> MLKCSLCYLASKVTAGNAKNQAGHPRRKAKLFHVVPGTPVTPFEKLKEQRRRFGQDRHSRLPEYRPGNNVRMDPNTYTLYATKKGVMTIRESRINPKYKWLDVEPDIQKVYRSRELRRALQEREMASMAVGENSNYRVELDLLLEPDWRERVMHVPKATERFKDPNLFTRGVVNELSPLDRYSYT;> MLRNTDVRLFSTFALNPETSVAPHGPPRGLVNRYVSMGLPPWAAWCNKVNRYSLYRMSGVTQRSFLPKPPQEMDVIWLNERVRERVRTSRQVQNVYRQLKYPYVKTGIHYSDVLDHWVQVPMVEAAMFEVEKDGGFDNFILKRSGPELRSTYGERIRRHILVRQKEIQKNFVLQKQAQMLVESMEKEILPMEDGKKVEEVLEKYGIDKEQLLRDIARAAVAKKQQLASAVPQPSHVEVSTN;> MQRNLTKLSAAAFYEFVDNNFLNNKRPPVPGGSWTVEVLRNKSLADLQHIWFLLLKERNMLKSMKEHYLRHQEELGAMPAPSRLKMIDESMRNIKRVVKERDEEATARAVEIFKERLKRGIYRYPPGPPPPPGAHDKTSVVKVELSCYVEEERLRELFGRYDVFEPHKGIVRVELKLPDEVLKQKEEAEQLWTQYMAECSDVKAYHQWSTAAPSAYDYTEVELAPGIFANDAISDKGGKHSGDTETHEGVIVAARVPVPPPKEKQPPPKNPLERLKAERRSYLARTTIQLGYFPNVTLPPPRYETVEAVPRPVHPDEIEGPWEAYITYDREDGLSYAQSLGITTIGVATVLGLTEHVREPQPYAVVDPVYCEALRRERAREETLMKWPHVPEWKYEYSTYTRKHLADIVQYNYTNVVDYVDREVLLTGKSVWECPIHIDHTCGGSKTVPPHAKKPVRYMDAGIANVGVTDI;> MMRRMWVPTFSAQQQHLHHAMVLKMSTYASTPSGNGVTSAASNEEMNLHDAAAIAPGPYRRVGNIFIVHCDDHPFKHSWEVNRMLRELRLEFKGQTTIVPDIPQVRKRIWRVRHIVKVDVLDLDEAKALIGVPEHISFTDLASQLPPSFGRVKAVPSPVIRSKMNFMKLRRMRLRDVLHRDALELRLLELKRSAMKNAEQQKHAQKDERTDNKEGEKC;> MVLHKWAVVSRSAPPPRGLRPIARTIPTHPRLRPVDYKIPYVLRTFIKDRHTSEVQHLENRGMFAEELSIERSRFPRFHSTFTIQTDGSLNEREFEFAVPPIVTLFHDRLSAHRERQLELAKIGKLRKERNWETEQKGEESVSMACNALAFPYCIPKNMLKRSRVVDPLNSKSSTQGVTSGGG;> MFRRTFFTPMIAQPTLLMLGNKGGTPKRKKNPMQLRRKVYGLHFKEKYLKMEEWYYCPLCAEPKKPGEWCRREDCRQIKP;> MLSSTALLLRGQYKTRLKKRMVGFIPKVIPRKIKNNMVALRSEANTGHMEGYLKTETERLDATGRKVQKVLWDPVLQRHCLFKETKIKGPFMTKSAIAKKVDFPIGGAEKMLKK;> MGSEESNNICAYKRTISLAKIYIVLLVKTAMLRYSRLCFPKMGCEEITRKARRVQLQPTEYLAQHRMQVWQLRFKEMGPPFSRVWVALGGKMRRRRVGRQVDVKDMRYYWRPIEPQYQRLYMSRLRIRDHSNKLRQPMRLRATNADIGSGSSSIEWERASNRKYGAMLAPPKRQDFEFRVV;> MRGTTKPMLFLCSTAVRLNFFPLGLSAGPLNSHILLPRNNFDGRTTHGMKKIQGQSKDPQMVMSRDELKLRCEYCRFEWIHDTLCVRCPAQPSHDQREMWLHSTWMWGKQQPYKYYKYMPAVRNPRTGMPMAREDARSMNNERRGQGLTTRTLNLEKERRGISRDVSRIGQYNTRWKTRFPFPT;> AAAAAAAAAAAAAAAAAAAAAAAAAAAAAAAAAAAAAAAAAAAAAAAAAAAAAAAA;>AAAAAAAAAAAAAAAAAAAAAAAAAAAA[2x];> MRSLIAMRRRFVSGTWTIAVSTQQRHRSGSGPGDKRIRTDWYRCYPSLMREKDRDMYHCYYPYLFDHGDKMSLYPKIPENPREWQPEQLQTTYDAIREDKYDAFIRLREKFPELYQDTRAWDNPPPFGEFNMFYSVRFGMVGVKAFTCKDYDELGNQFDCTAFWFPDNQVVKHSTRNGEVGTDKVYVGAMNVPVEFHKPHVAAFYKAAGVPVKHVCAGFPITPDAYAPVGTKLDVRHFKPGQEVTITFQNTDYGFRGVMFRHGFDGGYVWLGDSRWQRRPGAMGTEGQKRIYPGHRMAGQTGAAAETYQGVPVWRIDYKNSLIYLPTLLDADVGTYVRFSDTINTKGLTLWNEHRGLPAFPTFIPPEDEDLSKLATDECQLKSPPLYMYFRDEFPATQLVSQADVEDAKSAKPATAPPKKKVYDMKKYYEARKKYRQSMQKARKYKLMGLRTKAHEKQEEARRAKILKYKRMK;> MRRVSFSVVLATFGKRHSSIFSPRYDWRTSGVHDIAPRDEGDFLYQGPQHVLPGAHPLPLHHPHNTITRPVISPYIPSPQRSHPYFTAPLPELPHFSTTKPIVYTYGTMKERIIAPVFNLKNEVIYTRELDPFIFGMYPEVEELSKNLTYWMVRCQNFASKWDYETREIWRKAKKNWPNTGMGMPRVGNRKNHLYTWGGRTKPSKPWNMLMPTMDVKTWSKSNRMMLTLKMLQGRLQVVDRLTLEEPTQECYLELCRNMSWDVRHTGGGVLFMDGGSRITPSSEFDRAFFFGSFFNGRNKIVRPTVLCDEQYDYNKTAAKQRMKGPKGAKNPIPINRFNAYDAMKHDRLVITEGALMQLEDELYEHKLQILPPHIRNQLPEYGYLDSEALGDCVPSLKTIQMEAAARTEEAESDMYKSFIDNPYNPWKDNMDASYAVDGADGTVQKFVDGKKVSWSMLS;> AAAAAAAAAAAAAAAAAAAAAAAAAAA;> MRRTVVQRVAPWVPPPRHDIKVTMPPPPGGEVGGRFGVSQGYSDRLARTPYWKRMALSTYKLRMMENATRYPMSEHRPGEYDIRYLPTPYPCTIRNRPLLEVGEPRQIPSIRIPVIFLVNLFDEAKGCWFGRRYETVYVERQFMREELMPQRYAIYATPEAYKLLGLPVVNHHTHEEIPKTPREYEKLLERQRYDEERWKYTIEYLFRKYEDGPPELLDRPEDGWDGSEEIALSSVAGAGRDGVVSQRKGPVKQRKARKIKLF;> MSPASPLPVAALSRLRITHRSFLTRSRGRHVCRSAVGVEYRPEQQKKVLDHSYARVINAEVVHGDEQKFWGERRTFYTQRNIFFPMWDRCAQALILITREVPRVPQEMAFRLMAVFLKLMLLPRLMMNTELMLPMWIASNAEGAMAAAKDGSKGKEQSSKQQGESKDDAKKEGDNTK;> MLRACGVLQLRARPKTVCVEPGSNRLPEALVVEKARDIFGRPEFPGKRVLHNWRFFIKAGKAATGPPVGQEFSKLGLKAMDFAKVFNDRTKPHFKEDVELIVRIQVYFDKSYLFTIEPPPTAWFILRALRKKRRETGPVPLRGHYCALMTLEMAYEIAKMKPLCWGRPEYPLLETRVRRVVGQARRMGVCFIGVDTPYSSPVKDMTEQQYTEECERYRRIHMEQYTTLRQRELEEAPLIERLHRPNMSPLTDEQIEEGLRDPCLLDTLWRASHPLSPYHRDLRERELARRYLNARGWVKDMTPEEMRIVFMNYRLPEGEKRKQMDEAAMSGEVYWTRDGAQL;> MQRSTRIVMAPFKSVLRRHKHHPEGLPLYNDMSKQWLCREGERWWLLDARGEQLPRVAAVAAQYITGQHRPDFTPGMITGDHVVIVNIKDVVMVGDQWIRVPITWQTAYPGGKYRIRLTDMYERDPCMLMWWFLKDEVNRHFVRKLKTRIAPLEKAWLYEDSIHPHADKNPRPLCWTDPEVKGWKYRDPQFIRRWKPNEFMH;> MLSVSPPLRRYRLFHPRREAIPMHMCPAKTIFPLINSNNLLVKTRNSWEDFTGRKEFDEDHPLPVVGSRLNGRTTQHKWNHWDQYLNPQITQSIKDLTPTPEYVGMRCGHNMIKMGWMKIGGSWKYSRGYNDRRRVFARGQWQERKMTPRFMLAPRVSAGGPRNRYEGKLVFSPLRLSKLLWAIDTGRINPNEVITLYHLRQANVVGEREIVWPGFVLISNGVRRVPYPIHIELQNASAESIRLIEEAGGSFTCVYMTHEGLYQELHPEEYPIFMDQELPERRGLESLATNPSKRGWLTRWYEDSSKYAHPAAGRRYSHYLKPPTERDFPATVEEYEMVKHHQKWHLNQPGTGTLLPWHSYNTADLVKRAAGRL;> MPSPFQQTLLARAYHYVHPKTGRPIRQFRRYGDPRYINNEAALIRGQWGLITADFGMVTQSQMENARLAILRRLPRGSFTLTMHTDYEEFPVVKKSPESRMGAGKANIHHFAFKFTTGVPLFEIMPISARRLNQAEAEGIFLAGRPFIPLQTVVVPQGRVDEYHVFK;> MLRITLLVVGRAPPVIGCTRKARYAGIDDNPTITYKPWDTTEPLMADYGWTRGKLPKFRARSPFHRQQIARRMVTEMIRKDYCIVGGARAPALRILADHVVELAKAGDTDSRQQLAYFLHDPLMVDKAFDEYPRRFKDMNAKYAMMTRLKSRRRTDAVAMYFVEYKNRDMSDNHKGEDYSAGPERFFLPPRIVETEKGIQRPPHMQMAFDRWASKFKTEEFHHWWRLRHAKLRYWGVRNVPHPSDVDPLWTEKEEEEWHNEMLANTGEYEDLDLDDESYTAAGEGGEPSPAGDGPQPQRVG;> MGYTRERTNRHFFVARANAFFSRLPIARVQRSLAMEAVREGRMRPWKYTKEQILGAPVTCNFEYNPRPVRLIGTVMDAHTEETSIKGGLKVYARNEETNMMLWIPPGNPKLRHEVTSTKGSFQHYLDERDKWDEAWITGRARMK;> MLRRTVCVQHYRAKLELDRIRSMLRGRARLERKVGLKRLFFLMRTQTRYRVEQQAHWERAIVRKNVDSAAREHGTGWQHLRNELGRQNVMLLPRSQQLLAQYEPLAFRAVVELCASRIPPPPPPVVASVPEESYTLWPPASHDNSECASTDGSDAPHGQQQSLSHPAARVELRCGVERVLRRGPSGLGNNVNELIDAWKEFDVSPLRKGEVNK;> MPSLANGLRCPDALITRTLNPLLNGPKFAVIYCGNHQYKVAVGDVIAVQRLRVEIGSHIALKKVLMVGGPRFTAIGRPLLEGVRVTAQVEEQKRMRNVVSLFATPGRRHVRWVDAPHAATIIRICEIFYSPNVVGELDKYKGELLETFTPGQHTNPVYPVDDGYDVFRKKDKEAMENATTFLDLLGGV;> MPRPAPRFAMGHMLPHRSNVGSQFLHTQRHGSRSTWYKKHYFSLRPFAIQRHHGTTPRILLDRSLWKSLWITKLQLPDINRWERVVNSRRVTEDRYAFVEEEGVMHKVNWGLYCERLETELTVTQERLPQHTLLMKAVPSSWKKLDIDISVIRGLSLREAMAQCKLSLRKGHQIVFRALEMAQQGAEAKGLDKEHLRVAHISCYPGPTDKQIDIRSKGYYAWKTKKSSHLVLTLAEDPEMVLPDRTCLPYSSLMSMKRAGLSAQPTVIDVPAITADGI;> MVVSLRRFHSYANSSRGGATTCLITGGGKGHFALTVSTRGRFYRPLVDDGINLWRRRMGRIHKGWRTWEYQHTRPDPRPFPDPPVNDYFGRSRIWNPIACKLGYVRKKADEWGWPNKPPPPTGLRHSQEFFPFFFERYFPDAEVRLLLDSVLNNETKRPVFQIPCSMSKVELVNYLKNIYGIDNVVRVEVRNRRGRRYKNEVGEIKMMDDYKVAVVELDTPVSVELKQIKGTEDTSDNRPQERITQ;> MYARFRTRSKFYFRPARPALAYNVDPNVMRRPKVKRGLLKGTYSDETVDLRDRERLELLESMRHPRERDFYQDHTYHNQWLRRDLEKHQKQQLAARYKYFAPDFEISPWIWYPGDIVEVVSGEGIGQRGTIIAVIKYKNEIVVQNINVQDVVIPASESRPEQIVQREHPISVTRVRHVDPSTNEICNIEMVKVRNKETGEMEEKRMSLESGILMSIPPVNDELEVGDPLKDTPIQDADEATYDREAEQAVLVDKRLEAMEEHFVQSLKQSYEFHEPLRRKNAEDMRQFQTDVIDMACAMLGERLLDTVNASDTSSFPAEWQEAIAMHVEEIEAEMEEVAAKEMAEAKEGGAAENEQHDDDLDDDEDELDTSEESVKHV;> MVMRRCSYNVHPTWYMMPLRAYHMPGWKTKVSTKDVRTREQREADRKVRQIEKLPRPQALHDFQYPYEKTVLSDTMFQYPVYENELDTPHLFNITEPPDFFVYWNVSDFERTSYPPLPEEDHRLLLPLSGSAPWKQHRKRSLKYLRKHEILPNYLPHVRQDVNLSVVFPGVYATRARLCEETGEPLPPPPPVSRMTHRNFWMTAHCGNYIELADLQHPPSIFFLDTVSATGQGKAVEKDATEEGSDEVWYTLIIASPDYPFRVPASVDASTQRGFFLNYMMSNLKGGGNSTVLEEYESEQRQNNQKRQHLEELVRNPAPIAKEGDVIVSYTPPLPTEDAGTTRHICMLFKQRSYVSGASCALDDSKASFAARANFRLHAQHRDGIPSSSVEMLSRIEQVLPPDPSAVTFFQTKWDIQVQEFYESRGMLEPAAPLDEEIEAILAYHARKPSELRVRARHRPDGSTNVGDDPNFWAQAEPTRMMDGSMLSLWSRRTTLGANGVPITYRR;> MVLPRKLVGQCCLLLQKKQTAASYMANAGKVGNEEKWAQAAMEYLHEKRHCNDSRKRQHDVDNERRMAFAFDRYCSVNEKIFTERLSRLSDRMTEALETIKQLGMDHALEEALMLSSEQPPLNFRRPTLTPPVAGYEPGFGLDVPQLRSRQAEYPPVGRPTDAMEFGEEKDPSFPLVESFRVEDLTTQCLNELEERHGEIREAAPTTGVEGEAWEAYVALQKKALARQQLIFELCNNGELRERYDSDVAFRQRVWEERGMLPLEIERERLHEEPRHYAQEPAYHPFRKM;> MLRCSCACRRGVYHNAPSVYPFVKPFHDTPYDQDRGRHDSVGQRYRKNSWPEWMDNGADGTGYGIGLHRTHPLSRLRGNLKRSPSHVPRVLGMMIQGVWHKSGVKLYFRGGKPPNPSVHPYLTGEPCPLYGWKVTDESVIRQFNMPSIDGTNFRYKPYVALQERKIMGVQVPSDSVSLASGRTTESKPLAKRLFFWR;> MLRLCRVSLRVQSHQKKRAQHPNAGTRFGRVYNRGFIRYGFGGFGMSVYTPKKDRRFRVQPLPSLHANSLADDTPLVTTTRTLSPNFRAFALQDGGVFFTHPSHEQVMRVGQNILAEETKATGMTSMDTYVNSRIQSIIAENTVENVALSHWRRRHMWNLVRTHGKLQRHWGVSDATKGARSNIYGRPS;> MSRNGELCLKKVIISYCPSNGAPNTRQFLATHLPHFHAKYPSVSIDLRPRLWPEMAITGVYRDGSERSYNTKNLSPMGIFLRLNNLVSTANDYDQPFCASHLHFQRRSVQGTWNPWLWNYETERRRTEAPQWRRKLSEKEWDYYVGQYSAQMKQEEDEIQRRVADRTCVQEQSTREVQERWKRHVVPRMQTDLEFNLSHFKRQHARGQLQQRPVTMGEYRLFSVPDPRELGQDAVDTMRRRESHNMEVWWRKRKEQLKPP;> MRPVARLPLSRVLSGCRGFHSQHRTPVLPQVPAAEVQQAASESKVRVAYLLHRQPVVKPTPHPLEMEMAFLLQREHQRYSRHESSESATHFMAQRGQSIDALNRTDPRQIQSNFFGLELYQDAMRVVLQRYKPERRVTPRDLWDPATYGSSNANSNASSPPTRHSLHRKLDDYLHLIVRDEASGKWTVPQTELRGRETLRMAAERAIATDNGEGLDCYVWSNAPQATVPNANDGSWLFIYVATYLSGRPKFSEFRPKTIDHAWVTRHEMMQYEENFQSPELVRVLLDISADSTFES;> MLNRSRLRRVWLGGTAANTSLGRDVMPSTGKYINIVSPTDVAANISAGAMPPEANVAAALPVPRIQYSKWNRALRSDVYDELLKLPLRYKLHDFAKLCPPQRCQEEPEAVGVVGRDSAVGYLPPLGPADPLDTIPFFVHRSSNGVLPGKVFSMHPRNLMPAFYLRIQQVEGDMFRFEEELLKIFPTKKIFVRSHSIYVYNVALDGRMVLHHWLLGLGF;> MRLHTVRAPIITRAAMRGYSEARSNYDGTSLPAWPAPGKKPTYPAALSELRLPQPRMRKTRTEWMYYHGHGGCPGKYGPSREIADFEYADGTPASISGRRFAFKHHQDHLLVQLIRAAATVERYDASGLLPRIPGTAEQRNWDPAIPLFLDDVDEQGRPAPLRTAGDAPGTMVSHVCSRVVDERMGTPTHTPNELANRHEGETLEANTMFATNDPSAFVSDTVKLRDDKRPYWSRRRWALTDKFLVPKSPKPKNTIKDE;> MLNPPKHYSVESLRTVGLLPAQLALSRKPRLRPHVGNLKGLVYPLPYYAMWRGNHNKYTYNKSTVCLWGEGDTRSMYHQHYAHAKCPTDYGRGGREFEYLTVKRGKMLQKPLPRVQYVAEGSKPVWLFKSWHTPLSSPSMWEREVQYAEHTPEHIGAKRPLAVVAPRTMHRYLFLMHMEKVTITVSPLLFGYGHTIQKAVLDFYRRAISARSPFPKDKVFLFYAIDHITPRIEVTWLDGTSYVPPVLEGASSQDLIQMVMEEAWLAADRMAAEGRVLNPLAIDDYKWDQLVVFKKVRDKEASKGGGRKK;> MLRHCTAHRRYRTAWRELLHPLPVRARKMEWLKRDAVEENEEILRRPYYTIKSYALPPAVGRQESIHNSNNIRGGMHSSHSLDLIMRQPRRVKTPEQLRALRDRLRFIGVTGPMPQATSVSTKSYTDTYGSRLRPRYPESWDTVPPHQPSRELL;> MLRGTRGFLAVSPGVGIAPETTPVKYTPMMLNIQNMMWWNGKRNLYRATYREKTWYEISRTGAFTKGRRPVMRQKYSREALQAALAMVPPGFEVADVPRPPQRILAQSEGIVGRWYSNYWTLHSMRYQCLLAGVEWPLGERQRPRTNYDEPFFFADFEESKAIRDYRSRWINVNRSLVGMTKRMKEAEEEARYMQFRKLQDTFWSNRKVLVNRVKSMYNQGARTSAKDMPIKTINIKAFLSE;> MLRRFALTSSVALRLRFERDSGHNTVRYRPIPESMQPKHLEDNFTPFPLPKFDESLEYGPVRLRNIPDIEAAKERRRGSRLAATEVLLQETLQEENQFATSGKGDGNMAIAITERHTEDVTTPAADSRFPSQTMSPCSHEEEMRGYVVSRDYPLIDRLHCTRSIEELVAQFEDRPQIESRVAALADMASTVSFRSDEELLRMFTAISAPFSVDGRGLNFLTVKVSKFGRPYYVPNSLLPAYVNLVDATTIALVREQPWRLSASPALFIQVLQFMALIKVFEPNKWFTFSDHAPSNRADYRHAIGVNHSTAFWGTGEELYDFMVELLRVEDDGRIPTMLDLCTREQMVDLLSGFCGVMPCGKAVGDVFKTITDAFLRRVRNDISGPWSAHDWAIVERMYLVTVLCDAGNNEILQLLLSDTASPRGPDFFAAVSRTKDTPTKKRALCLLQEAIDNASAKADKVTLLGLLESGSEFLLSLVDKGVAHTFATQNLFDYRILNSFLHCSLVADRLRVEQSVITSLIPSSLRDVQVQMLMSNERNALNPLTSSLPGNSGAIATAPKLKRPLMTMLSQLEYLNSIDSVFILHSSLMATSTDQLVSAVRRLPSGKDSLIVTMSCLRALSVKSLTSPSMKERIACARALEIVSYELEKGRAVLLPFSEEILLHDAGAYCDEDLMLWTVAAFLARELPLVKVHTLMHSNCTARTPYRFLKGGHNLLVSSRSLYDKGAPLLSSLHSKELRLVTHNVRLRTPVRDRKCTLQYYNPIRARFVYRRDKPLFDKYHVTARNLAPGFSRGALKHDWRALGVYTPDHPQVPYHPLQTWMLGETTVEAE;> MLYTRRLMTTGGSATADGAVSYSKGSYHIVPKKYTVGKRIAVRSYLDRNRTELSDRTYMPQKAWFEPYTPKKFDMEHQRISHNFYNLETKLIWTAFDTPELIGILLHDETIKGAPHLYDAEFLESAVHWTRESRYWRCIGITKPFYNKTTLRAQCWHDRGLQVGTLVFSQAMRDALMDLERAVRRKELGLEPNYVWDRWGPVGFIDGARTDHLPRFAHNPYVDPDGVEVTEVDIAPFNTHEQIKERYGAFIDPDLRPFEGVFRSSSSSSSSSSSSSSSSSSSSSSSSSSSSSSSSSSSSSSSSSSSSSSSSSSSSSSSSSSSSSSSSSSSSSSSSSSSSSSSSCDEKVEALRLMENTRHDAARVRTFYEEKCGFSDFMRTPDKVITAAVLCYLQELQRICTETDWGKPLARCLTDLERVNVMGKDAFLVYRHIEDAILDKKRRVWATRFAGEANEESTLDYLLENFGRRTEQTRNVGTTGTEFDREQEPIGRQVQRRVLDSDKASKLAEVRQKRGKMWSNKKSVFDSLHQKQLQNVTYGVH;> MLRRLAGCVAFRKNVVRPFMNSTALLSSPPAAVSAPVIPKSGNEGKDYSVASGSVDTPVLDQLVGYYVNIQSRKMYYKDFLRIEHQAVRWAFADIRKNSEALAHGLLQTGLRPGQRVLAIQPCNCETFVLQLACAKIGALLAVVPHHNISADKLRFYLNEFQPHHLIAREWIVVPEVKQGVLVERNMHFWDMIYNVIPELGLSYPGQRFQWVHSQEFFFLKKVVITDHNMNLLGVTPMRKMLVWGPFSYYEQRLRRLSALLHPDDPILALEDPHPALEDKLHITYSHRNCINAGFLFGNLMGLKAESRFGVMPNHHVDPVGAIVAPYAALTTGAVLVHIHSDMFTDDHAINGIEKLCVEEVVGMLGKKSDFDLLLRHAGNFDADQYEHLKWVVLFEDASEPTVGDEYLQKLAKELGLEDVFVFRGPLESAYMVMWRSLKRARWEMVPHVEAKVVGDRGTADARILAANTRGNLKLKGPHISAGYYNNAGLLTELVDERGFCSTSREAVMDERGQLTLHGTQLY;> MCLKRKAPHLFCFCLWSIFLSFRCFCFRSYAIMLPLLSFPTIQISIFLSFKLPITTFLLSPCFVFVFVFAIRYCGELTLNAQLVLFLLYHCAQTQRGPLKEGEMPICPGLCGELAAVPFRVFLGTLPTLAVEERFLRQLQPVFAWYSSRKRVKEQANEFIEIDLASCDAELLLRYSHIYYVRRQLFDELIERQMTLLDSGKAPKMAEPSLLQCLAGCNMTIADRLQLEIRQLGAAKRAASVPGRRELDPVARLEVYDYACMMRLVEEDAGAVGDAEMKARAYLPREVIESKLGHLTQLLLGSDARAALDKKDVKLLNRMIPPDYTRVGCVEKLRPFDVTAYFRFYGERINNVKVENYFKRALWGHVYRRFATTPSFLSGVSTYWARHSGLDASFTTTTMPQEVAVAVCDQQIQFPAIKFRAQYVYTSPETARQLWRTDAAVPLMRLFPLMGSRTAEDLAAGVLTDAFWMHLGLSEEENLLQDSLLLKVRRFVDEVGDMYETNIDSVLKRVDDNFKQVVPQLKAEDLQVDAPLQDGEGEDTVRETVAA;> MLFRSVSCKNYQRGGWSPGSKHQKHMTLNPTLYLYRFPGPHGPGPYTMKYWWTLGCFPTGMEVPFRLHEFLSTYQQEHVPVEVEEWLRCYIKDPLSELVNASNDFFKAVEVYPEVESARGYKTLQPSIAPLLVPMKKFEEQLGVKISPVGLRSVLSNPVLKDRFLDDLFDYKSYVEKGGSTPHRRLARSRFEGSLSVLGECEKCLPEQHQVEISESLGTFIGATVSPAETTADDERSLILLLTTISEGCINAGNYSDAASVLADALMFCHDPDSQATTHANISFASLLNADFKGAEYNGREAALLQPQVKPTSTACARGYVGWAAAAAYQDDFEKAEAIVKDGLTLYVGNEHLEKLANKLQALREEQPSVYKQVPRSLRESRSHLPSQQSRGLLSGSGKGFSNEFDWVEFKNKLYPSKMDPRNNEMGSVFRRVGDLGSFISTSRSMERL;> MSRSAFSSRGALLFSSAPLQCQRRWVTRLYTSYYTGVLYPNQLVQPKQRLPADVSVSAILQKRSEPEAAAERGSNKGDKVDVSKGEKTPRVSWDDADSTDVMRVDNTQQLKEAPQVERPYVPLGEVAKLELQGDYYMEGGMFQEALEHYGVVAKAYNYAYPENHAQRIGIRIKLSAAFRQTGRLESSLANIEEVLRMLDASTRPSLELICEALLELGITREALGMKREATEAYEEALEVVNSFHNWGESHRMLRLLPRLGRRFNYNFEEKFVYFSPFDYDRTFALVDQCLERAETIFNEIGDVEGAIRVLQQRKEMIDKKFFNMRDFAGRIHTMRGHWKRRAQHLTNAPTPDELLRYSPTIHQVHRDFKYELTAPIGREKEVMPGVNRLVLDMGNPYRRRGRLSNKMLKDADHKFANYVRQKEYNE;> MRLARTLHHVASATTGGGQMLEGLVNDGPEVAHKQHASFTPFSIQPWQARCVGASRRKLLPQMLMYHGARLGPRPLIILDHSTKGEAGVAEAARKYESILSQLSWDYGAVYIPLHAQCTDSSKDLLEQSCQRICAVMDALDVRWTHFLTYSYGALVAVRMASSQEFPHRVGTLMSLDTPLVTREFLRNMEQREDIAKAERDINVPEDGLAFAKQALLSSLEGPLPCPAAEDESLYRDYLFDPNRIFGAGGLVRDESRYVPLKSLLGVRHPVQLIVPSANPLSDAAAHSEVFGHRRPAVVKCCQRHEDLFKESAAKEVAGVLGAWMRRFEPDCFISKRYEQAANEMGQLMLSTAQVSSESAGKGGGEPRKKKEKKKSKA;> MLVPGLSLTRRAVTSSCCRPLHVVRGFSTTCTLFGLEQLQDVPTSTSRRPTGLHRGPGKRQTSEREAAQYKFIRRWELQMRDEWDQLEPFKGLPKPKRQFGNEAAEVIWPYALLLERVVKVHPFTKSIYVYYAQRQSTARGKLAAEIARSFAREFLIPITFHNSQVYTEAEMLLEYSETPWVVLHSLDNGQKPRILPVAPVEGTPAHTAVEQLLAEVVQGCEALGASVADPVTATRVLNERPLQNQYVRVDYQWFGDTPDERASHLVRWEFEPEQIEPKIRHRTRHVLDWLNYDGNLPTHRAVHVNAMREKARQKAPRTVAGPRTFYNSAGSRANARSSRFGGQAAVGK;> MLRRSDLLLKKGWTHNPGRTRRGGKNLAWRPKMSERTLEQFVPLHLAFPRRHPNSWQERQFHLLGYVKWPKEIGFYNAGDNFELTPQAAYRIYKQNCDETFWTRLHNEKTIIHLLPLVEQDPGTNMVLVDDIFRHHLKRFGADHYIYNAVMQAAAFAKDFPRCEQLLAEMRGLGLEPNAQSYVNMMLGARLTGKPRDQAEAFFREGIKTGAISAVMRLDTEFQMWMNQLERLGSFKAKVGYLSVNEEGASPMPRDMWALWGWHRTEAKFISRKQMISEQVQNRVRSGKELVGTVYQKARRQPWAKYNGMFPYDYNGPARRPAASFVDAPTPTHNAEVCGTAYA;> MLRLSSWNLKSQHHNVLRRSRPHIHKYRELNRWQRQAQGISKWDQSHSHRPLPYVERFNPESVGLTRGTSAFAWKWWHTQYPWLPNVPPEAAQIDEAQKQERRSHRPPAWDDEFAKVVLNMNDAEIREYLMSKLTDVIFLETQRDGYELRRLDFEGKPLTSLPEPRIIENFVLEEETIRERVIYQVVEGVFRLSPTSADRRELRSVANIIDYVLTHVRAARPTDRERRQERPITSAALAVMQKCPIQPQLGFVHALPHDTRDALLQEWERMHHLDWQFGKAVYTPRSKENVRGNLTWLREDRHYDQRMKFMQEVESGEARAKHMKLIAEAAGN;> MYVFRFHISSFHSFLVNFLQPSRGVGEPSRLLHHLETHPSYMRRVTSTAVHRTVSSVLSPALLPSFNGTLLLSVCFASCSAAPVRNLYKRLGLDHKATSEEVKAAYRQRALECHPDVVDDNQKAQAEVDFRAVSEAYDVLIDPQKRKEHDKALGLERTVPPAKKQQEGEGVGCDSKGSFNRGVTRPRNRKPFVRGDADRNFREAFHGMSLDQVLFRERLRQRRMQKQMEEKAKSSSSSSSSSSSSSSSSSSSSSSSSSSSSSSSSSSSSSSSSSSSSSSSSRDPQPPPSDYMPFRPFHGWTVPNGVRTPPEPTLGPTAKVEDVKDVQLAEPAVGDASHQRKLPKHFPVVQASDGSSLLREETIACMERERRLPHNMGKLYSYHRPY;> MGASAGLIRRGGGVFPDAVSLTLTPSRRVYGGSGRGDLLYENPDARRHSGRALGVLNGVRHSSQATMPESGQLYYRKLILHSRPPNGSCAGLQRHCHDTCNWSYLIPSLHRCAESAISAKLWEKMCQLGLEDRSKAWVNLTQYERQRVRDGQNLYRYEVHQRLPLLEESIGWAQLDDLLGWFR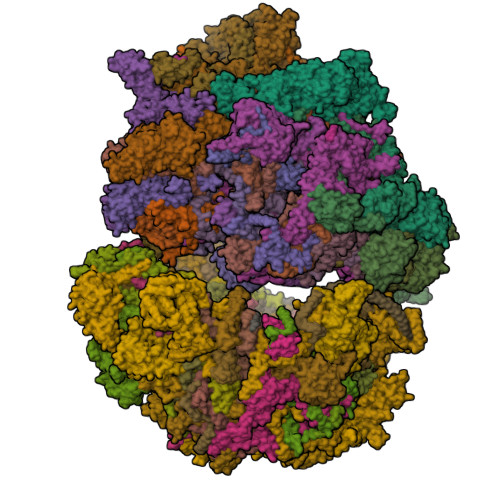SARRAWVRLPTSVTLSRESSEAGVASVVSPSSAMSCRLEGHADSRDTTPGRNQVFDTPERVEQLTEATVHRIREELQRLNRSERSDCEGSAAMRASARRLARDEELSRCVEEELGWHGVALQHRIPVPK;> MRPTFPALGSRAKGYENRVMVYAHRRHRAWYLPPKLAHARSPLANKSPDEYGNTWDPRTGVEWYHRLRRRGAYRHWPWARWNDDPVRQHQELSCRRTFSAAVTGANEGVPLWNYYAEVGQEYGLPSHFPLSFMAPFIHQYTSRAWSRKEIERHLKVVEERTGLRTIQQACDATSELLEWGEEEMGVVPHGLLQHVVMLAEDIVLQNKKKAYRKAAHERGILRTTTMERYYALPHLRTGPPMPTTLEQPSGEFPWGKFSTMVGGTRIHPLYRPDGFFKDNMYPA;> MCCLYTSDVFFWSSLVVSPLPRIVRCVSAPQIRSIPCGSGDFSVMKRSLIARWQSGVHTPHGVVYRGAKMKNWPEQRIPENFKFTEEQRFRTKAIPRDVGTIPRNFVLGVLYRHQPCEVGGLWEHCTNDPEIVLDSKRHLREVLKQAREEGFVTFERDAISNEWLCFLTRERYEEVQRIVTAKSEAVDSSSSSSSSSSSSSSSSSSSSSSSSSSSSSSHARRLEEEVANTTRYLRRFQQREIDYLPYTDLNGKVNFMWWYETRDVQQRADEVLTDSSSSKALAGEEEHKAGSQLEATTASTS;> MKRLFPSAGVSVVLTSSSIVMSCPCNHIFTSRRAYYWPYNEDFVPEGAETSRFQSSGSPGTRRRVLQEYALSPLFGARVPCCVVGTLRTAKEIIVLKRDIQSLLCELMELPQGSVTLGPLQQLREMMLYRHGTPLSPRLGDERQLNMDAYARRPIAARTMMDVFLAEDMSLDEIVNFGRLSLGKLQIALNNLRKENAEKSSADCEDGSAVEPAQLLVDRMGISYCEIPSLDESDYVFAEVGGVAVTDEEAERVAQRWAERCE;> MRRCAACLTSLPVSSPTGAAVGAPAAPLKTQAPSNRSLLGYPLRRAAAMEMLYGGICIQHLAQPPFPLRKIQSESLPPPSLQGERDDLELEVKDSTGNVMGYRLFPVNIGIRARTESVRVRSEDCYKRFLAQKHCAAAGVPLQFPAPSSITNSNCLATPRAASHFHPPSSSLSLFTRPADSQGGDVGRTTPADVAAYHPRAWRPYQMLKPMPHNWGPAVRSSGVRGPHMQLLQERIDKKGFGWKRKSRSLWQQDISTAGFRPKRYF;> MLHRTRLAQLINGRILQYFVPYERDEVNPVVFMDVTVEGDALGRVSVELFHDIVPKTTENFRSLCTGERGYSQCPLFYKGIPFHRVIPGFIVQGGDILLKDGRGNVSVFGFPFPDESFEGKAGKHLRGTVAMAHSAPNQNGSQFFFNLARNDHLDGKFVVCGQVIDGWEVVDRVAVLSGSSCGTPVSRAWITECGQSSGDKLEDTERALSGERALHTMPGKEVLDILSPRY;> MLRFTRLFREMAPELQLEYMPVLFTRTILGPQGGFAGEERLVKLEVARKYMEAGHAVTPTEELRRGLWCYNPDTDKYDCFIERNEEFLDFAARKRQWLDVYWRVNTGYLLFGRQSWGQGFLINCPLRKRDVAQKLWEQYKVRIDPRLIEFREKDRRTGIQELGHNWCWLYLPGAEELGINREVYDNKRVKVRIHVRKMNSMFALY;> MRRLGVFCRGQRNSPLLTRGIATGGRVTNEDRRWWLVHLECAPDITPGTFIAWLDCCGTHTCKKLIERNIWTIEQVAALDSDQVDELKYREGCLKMDVVWEHARTIITPLRQREVTGGVESELQGRIMELRKKRELERRREEILKERANVSEQREETLRK;> MRRCIPARGGFTMKYKKGTGLWDEDHVNDYKTNRYLSARATMRWYQEMERHQTRNSLNARRATQSHNNNRGLHHTGRGAFERELERRGVQVEKYPLTTTTGTMRVAELVILRRMELEKRAEEALAEQRGELQKKNPTPSEWYDESKGPLNPNFLRSMRSHYEVDIANLPDTPLIRGQREFFIGEERGNGAA;> MLNPTFSLYRKTLQSYPVPPKIRHYDRRWSGSRTNPYNRQYWRVIMNENYSRPSFWVSDFRHRYLMRTGTDYQGQVPSSPQPGLYQGFSDVHKLLANHPKPQRESRHLPVLPMTPRIVFEHANEKRIDTAKRMRRDRRRIEELKTLEFWGWYMKLQRVRGRWCREQGVSSRGVYGPAVDAAELWG;> MLQINAFKLVRATPFLLKRTGKPADTPDYKQVYLPYDAAPTERELERERRRFKQAYHGRMEHRKLVEVKEVPLNVYTYGKEGMSLPIAIFKDQKDPVIGPEWTYPGIYENKIAAQHWYTEELFDKESKEAFESPWQQQILDNQVKRRMAKVMFRMRQVNMKAVDLFQKERGSSRRSGGAGEKGKDGGGKK;> MSGAFGCGSYRSVVAGTQNVPRRMTFYPSAYELIQLHKAHREVIRHFYVRDKIFDNKFPGNALANGLFKFVPNRRENYHMRELMESIRRRSIWMHRIKQQREINAKVVENMEVKYGKKAAASMLCFTTPDSNAYFAPHRYQDVANSWPNYWQHPSVNHVVPKPRWRRHRELGGITRVEDPFAVQASDY;> MLRSRIPCVVVTLVQCRAMHGKPTQSHKVRTQHSRRWWTQSKARHLTAMPHDECKSRPHFPAYNEDVDRPMVVPPDAICFNCDKPIDAGDVNSYVWIPAGNATVPTPQGYFFHFGCFKCNRCKYRLGHNKFYSKDGKAWCIPCALGRDVRVPTRRWHTSYVNTHRTGSRLTGHFFPRHSHQMEFLFDPNS;> MLFTRCLLAVTTINSSTASAAGRLIRIRKKSKWIDRRSKRIPHNGKDVWQFGEQPSCALCHVRFRFKQDYEAHKESELHQNRLRWVETMKWWEEIGEPHHQQHAASEWEWFRQRVLPAKAAAMGLSEEDAARELRRAVMHETPRWYSRIQPPNARSEIKEPRDQRWPSSPKW;> MRISERAFMDIAIGTKAPRRIVFKLFPRKCPSAVKNFIELCSGNVSTDTYESGNRDKLISESALPQLTYKNSTFHRVEKGYLIQGGDIVTGRGTEQLSIYGGTFSAPEEVRASVFDKPGLVGTASSSPNAHGSQFFILTAKEANHLNGTCICFGQVADGLDVVQEIEQVPIDPSGFPSLKVSIVDCGVLE;> FKQGQGMFSHQLKRLLQKKSIHRYNWDPLPMYDPRKLVHASRHMDVETWREVPDPHWDERSYLVPDQMFYNIPVPPEYKDAYWWRELQARRVQCPVEWVSHRMYNKGDRQRYDFQDLAFRKKFEFSYEEVVKNAKDMRS;> MAQWVPKTAWKVSNLNKRYGPGYITSGFSSENTLGYTHMVHDSHKLREKLSSRKGIFVIDVRDPGERKLNPVPRSVALHHHDLLSGASCPILPQQKSAAELFVLASNESRGLNSAAALRRWGYDSVVQVDYNTLVEAGYVSRCDYATAGTKDSAEQAVSGED;> MFRPTTAIADSFKEHYHRVHLPRRLALQRYARQQSLRNAAKGNVKAEEVPYKYNRWWVNEEHEFVHQYAFVEDPEVTKAKRETLPPVTRENIWKEPQQTFFLPFAPYVRVVDYPKDPDAKFLKPVNIPRWKDYMQRTKPVIPRTWY;> MNDIYARRLAQATMFHQLMRCHGTLWAATQVTKEQMDYNFIREEFMRVNGRRAMPLLLGAAANENLHQLHLSHLSEHCAWGESARALAVQRQTPLSQRVAALGRMAETIHQVKTASTVQNLFNEQISCMEGISSFEEEPLIEGE;> MSSRFFQKYFIRCGNCQTIQRYAKGYKPIPNPILFDSDAHCRSYHRERRDCTGLTGTLVTCRCDKCARVHSHWTVMDFQEFLDAKLVMTPEERTALLWPGAGSRAEPSSGTSN;> MVLRGVRLRSVAVSCYGSSLTAATRCLSVRTEDFFSKEAISHARRVSWAPHTTEKKQGAFAKLARSNFGDPLPSSFAQEPYFEEEIEAHRKHHRPDVYIYKYNVSPTHFSLRE;> MYQRTRFLWSSWRDYPLGSRDRRGRFNMDEAAAALQLNPAYAAALYRPLNYTFHIRGQLYPAQKGRPSRPGSLAASQGRMFPLYQRNDRLDKELFRLNSRGLTTE;> MALFSCFRCGYMYEFAVSNSYCRKLTLRNDHCPRCDQLTLFRFMSVSGMVGNMPFKPIGVPGPSYATLWWRKTREGKEASAPLDAVCKSDRW;> MFLIHFVHYKTILQKYTFKFKHIFLSIDKYNSLFFNISGILIWLNIIHINIILIKYSFFILINNFEYLIILIST;> MFRLTAASQKNLNSWYTKGTMRGGVPRIYYAWMRPGSFTRRRFEKMRNPFVDLETGTSLYFRDTRDSAEAIAHAADSKGIKGMDNAIDLYNEYRIVPDLYPEGFQWKHKLNTEYNQWRSNTWLTPDLIPKEHRGRFLCNFQLNIVAYDMRVVKFSPKDHRQWIYCVLYVGSGKGIAGWGRAVAPSTQEAKKEAIREAFSNIIAVDLEQEGPMYPVRVNADGVRVLLYPARRIVANFRVADILCAFGFQHAGCRINLKATNNPKSPTHTVEGVFEAVKALRSVSEIAASRGKVPHSLIYNIYPYLEEIRRRKGMMAMHPPGKDGLLMPDRVVDNRLPDHLKRGYYDDVYWKDFFAGSDEHLNEPRMGLRGDEMRRRLEEAQTSPAPTTAKDTRRRTLEDVLKRLGKTTRDLGSIPIVNPRVDVGLPTHIKRNYQLH;> MVFYSFVLVMKPRQRRFTSQALREIGVAVYSNGGLIRSITNEGIMRPYSRFRDADNTPLTYARYIILQLDMGEEEMGKVDKIIREHQDVLMALKLNNLERPVGIRSGNKELQAAYFPLDTFTRLEEEINWSPQTSADIYTQLEMNWKEFSRTRWSSFLRN;> MLRQSLLSLAKVYGAVPPLGAAQGHRLLHGKREREGSLFAVANDVKRDERLLRQQLNALLEEERMPMQARLQRNEAVSSHEAVPQTPLVDLPGVERRRDLPADPITRLFFQHKGDHALYYGTYDKPSVQDDDRVQIEKRVPRRREENLYTPIYDFCHRIREATEQRKRFVVVPSTIETRGCARVMHDHGLVAGFRDFHNDRAFAVELKYFQGDSTINVIEPCSYDGRTEFEWSPKMMRRLLNTHGIHNRLVVYICRTADNRIIDHIHAVKENIGGRGLMMVH;> MQKLLSPRTARHARLFRLAGKLADSGSPGVPKSDGERLVWVNSHVRRDKDISLSQEEERIRELMMPLEVGENSFAANGQATHGNLFYFREYPMYPGEYVPAEHNTLSSLRDELRLDLTAQSLKEAWMRVSGGVYFQSVDEYYASVDGLDAEQIGEVLAALFPELNCYEAQALVQRTLECISRPVSAASRQLSRTITAEAVGLDNAPGHYTNFLEWMGRLTETRAFKTEHALFEFSRRKFNRDDVRVMFENYRLMSKATLLADSADSYSHFYTVLKDFARKVAGEDSRHQIGVRIDEAEVDPETGIAVGRGCADGEKYHFTALLRENRDHNGIITVMGKPLSLVLDNKAWLMEMVLMPFDEANLDYRDFDAHIVSEGHAMPSIANEIAAFALRMAVANALVKLIPLTRIPLKKSGLLSVDRRRERGQFPGYLDGKKVKRRFAKR;> MVRRSHVVAYYWSRYRMPTQMPKFDGPAPVAAPQSMNSTKTNEFIDPIDDKFPMSIRGPLVRPDVPEDQYVDSWYICTSMTHHMGDYRPWSASAPPNAFRFRPFNEFDAKGREYVQYMREFARFDPRKSRGNGQKGFPFRDAYLTKMNEANQKTPPPTLETIMDRAVREHHQHARILSPLEVQRDVGRLEPIPSYAGKINADRSVFPFQWKTEDWYEYEVAKVRNRRFVFENTEEDGIRGSEVTYKIVLEGFWDHHVMKLAEDVCMFLKDVGRQIVEEKLVAVRRLLQGGAVDPELLAAFNCARAGPFGGLDEYDKEEVANFLRSDLRRLEEQCLSVINRCNVPVPGATNIYDPHTSWPHVEKLEPWVRMAEFWTSSSDTSFTELEMSTAHYEFRKFFRVIICKLPFQSTEFEKRMYDIRHWLHRQTSCEFHTIYRRNVIHDSAVFPTEHDPATPTTHEHHRMFSFALDWQSAPVNRLSTDTVHEGESWDAVAQRLGCSVGELKDANAERETIEAGVVINVPVTATRRLTSFGATPLVLPLKTTSAKDGERIRTWEEAAAILDCTVEELQQCNGHAALTYQKKESEAGEFDSSETELVAPLSCWTSTSESEFSPVERVHANDTLVAIARRLQCSEEALRAVNDGITDVSGLDFVRVPPEARRPRRLVEPQLRPQAATDALLARTIAEEETFKLKSIPHLPQNAERFPHEYHTPTSRFPPTPSETPATQDWMAYTAKYLDKQFTISAEPAPVYNVNKLWPMQQIPGKVDQTPFEEDQTWLLHSIPVQQLEMHHHEKDLQDLPFINHEQFPRSLEWNAP;> MMRKSVTFLRRGKPRPRAGMFPDKYRRVPMLLKPQQGGQQYFNHFLIRSTNDRLTQQDVDNASGQAHSFISPQLPQMDWRNMSARSSEESIREEMRQLAENDVMQHQRVFNERMWYEKEEEHRMKARSCPEETSEHAXSNDGAVPPPRVLGGDYFKTRFGYSLVKNSEMTQGPVDYSQLDMWGEMPRYTSDMVFLYLVSRRRNTYAVAYTYEGKRILNTYTAGNRGLKGGDRGFRSEGSTDNGHQVTSMYLNDLLPKLREMRASEGRPMGRGEKVELVVRVMGFYNGRQGAVRAVQDRANEFHVRYFEDITPFPLNGPKMPRGVFK;> LFFLRMWFLYGCCLRFVLFVLCYYMSPRLPSSGNRRVLYAVFYLYNFVWMLRCFFCCFIGLVMSLFIIEGGGFVDLPGVKYYTRIVS;> MFCFSRGLWMRHIGQDVPKRHTHFVLESRLMYEKSFRDCWLHSVCRAISQLDEPLSKTVVGTHQKMLQRKVTCFQYNQYGLFKTPYYRLANVDRYHAVQGVAGTREWVPYVNVSYWTMNKMVRGGNLLVHRVHYTGWGTDSHLKKGGWEHRWNKVLQRNVLQYSRI;> MFVRSFCFLRKYGSKSKTPDLKTSFTKTTNFRKAEKISITTTDGEIVKGRGKIRRRTHSALKEAIGAMEHPAIWLWYPWRMNPEPPTPHMPQRRALKNVHGAVFNDLTPVQKKRQEQMLYGVNIPETRQMKFEEQHPLLAGALRKLEGQPKGFPFWYRKYPTRRHAYEYRFSIPVEMLDGYNDDVKKALSKGMMSIQEKQFAQEAMYMERYAEHDFDTTSPAVLAVKRALKCRVLRNHLLTNPHNNIIKTVLANTERKLNHALRRLRKVDFKKYWEIIRDHDVQDILQPPNLVTYRQGSYWKYDWNAGLAISTNLADVMDPRGLNGCVETGRSRSEVARDLGLSYTRPLHENEKKQLSHQAVYYERLAKFKMEQPEAARAMERERFVRKFSGMFVKMDIRSGAPDFPSTYRRLLGTKVVRWASKRHGPN;> MQVTETVLARAVIKRRSPQLWGAPGAPIIRMRGHHVVWKFQSYDLVVEHTHKRRNSDIRLLHYLGKHCPHPQKSLWSPDTPVAQDRHLFMLTTVDIDAFKYWFGVKRCRLSMKPWALLAKAGLLPPSLTQNSKIMPKPLFDKESLMRYYLANRKDEDVMAREKYLNYENSMVKTEEERAAERPVAPYL;> MLRRSLLAFPWWNFQTEHRQRCVLMYGGARTKNTHNANHRVFIKKYKRNAFPNRTRHHWAVSMTGVLSQRPRRMPWPYDLTSLIFNQPRQGSDKIGYVVGTSMLKTAVVATNHMVYYPKFNQRVSRTKRFFAHDEDLACVEGDLVHIKQCRKISKYKHYYVFSILEPNVEGRERLKLGLKAVPPPLFGYPVSRRIVKLNLTSTEGTQEKLAAAIQEHVQDAYRFSGPTPDQPRNRLADPVTFEDANNMIAPNAPAAAALDASDSPPLLDRGEYTEVEQDTRNKKGDDYWMNLQPKEKYDFKSFKKSP;> MNRTGGSIYAHALSQFAVCRQPWNEYIGLLTKQDSTPYHTEPQEKPAYRGRKQGREGWLFGQQVQLHYHRFPDEQLITNLSRWRTGETVGDIAMQQFRNAQPFDIEDKDPQGVQRPSPEVYMKLNYKNPATISRFLTRTGHMYPADILPLNPEAVVKLRVAKAQAIRIGLYPRFGNPFWFRSQKFRPKAYQENYDPTTYSTKRTVEHFAYNWVQTDRIRRYFRELEAVHTSGSASARGSGGGTTAEHKQQDQFYSPENQPISLHRNNISYMEDVGRSVKNPTVPGLMSTKGMKKKFHNLYSSTSTKRMGFSNPTLGIKKV;> MAFRNTFTTPGKFSTVSKNIVLLLIWRVKVFLRAEGFAHSLVMLPVSLYSKILLCDVKKKIVYFHCCTRKKSMLRRCPCVWPDGPTKSSVSIGTAFTLQKRFLKIAKSAFGFYLARRGQRKYPFLRRPHIKNTHSMNPSAPYFWSFMTAKSQMAFLPEENYITGDWTGKFFVSKRQVYTLQHATSGAKVRVKSFPSIFEFNSPSRWNIGKEMNTLTKPRMDLIDEQMLTKKQRLDYVRAGLLPK;> MLHTTRLWLGGYMMYHRKAMGTMKYSKWKGAHGGISHFYGRTPMVEEVRPNEPITLVDRRIMHYVHHSRLRHFQLFRSYQEKSNSTECKLREGEMLRRRWHRRLQKSFIAFMQFKTMKVLEDQARLVNTYGQAAVNAALGDPWNATDNVARERKSAAVRRQVRALPMVNVVPKHVATMKQIHNDRFNYRWRVN;> MMQRCSTSLSRLCFRRLLRTPLLVYSIPPTRDVPSGIAHCPLSCSMRMVTSSNDDEFVFDPTLSIQKDAAIHTAKKSFETIVLEYVPAHAPEEARQKVKSYLTQHPIDILITQPKVQITHLEDAESGAETKVSLSPCDLPEALQQARERGMNLVQMGARGDVAYCRIRRESTRILSLIHTELEALREQEEKQQGKGRGGVQAAAKMGELIDHTFRDAVDAHFVGWRSKKIVEDIRRRHPVKLTIKEFQSPECAIGKLREMCQAMQHYAQEKVIYHHFTSIVANDREASITFAPALPMAKSDSWKHIKYPGEKEWTNALRRMEDACRKSGRYGTYAKSNKLKLRSLGQTSYRVDKYGRKMD;> MLRRAYIQRRYPFNKRGPREHKSWKHHVLTEPPKPLQWRDPKVWTRDLSVMKSFDAPQWDLWQSRPRSEDMDEALQPFMDMPKSLKDRRYDIPWWANPFGAWYLQNILSLELLKLKSKTNAEKIATYRSYMRSLASGKDNTMSDDDVIRNIIKERWKTLEFGDRNAGYPCTFGDYIQFLNEWFKSLDEEGMQRLREHFDRRIRPLLAVMSPVDILWLEALTQNSPHNKEQLQRKIAFQTSLGTPEFFDMSKRLRYEINEDYKVRDELGPELFALWSKAPERWPPERLSKMYGLDFTLVRKILVWHHFKACYDACVEPDWSLPKRLFALEWIRDVRARKHGLFYGKMRFAEQKITFYSDRFLFRDLVNRREASYANVWEMDDPYRFLQTEQDYEDYWGDNYDVYRRMFPEMIGRTGEPVQQYGQMPIWAGPHRQHANKSEHNWMFAEIGVNVGHEALKKLELDPTNEKRRRFVIRQPDGTLRSAKMSEMRAWYWKEEWADFRFWAPQMEWGIENTPSQEQYQEHVPDTTDADFRKQRRIQSRPVKWFYESHYTRTGSFAGFQPLRFMQRRTEREVRWPDVINAAVQIQKRKPAAYIFKAIPEL;> MRQCVVRRYKMPKNMGVAPRFDTWNEKYEPWEHMKRMGRLVGTGFYIPPEWYNHFRMFPPINHNFQQEKTLNPHNASEPTQDDTSTLSPERVALRDELARKSRLVASEGMRYYNIFWVRKPLDTMEKEYYELKRRGVDHGEAIRKVLQGFYSGLAVKKRVAAIQAEEAKLTGRFITMREATVVLGVLAKLHKEQLTPHQVSLLAKEQGETTQSGAKLTAIVSRTQPHVNKEASSPATSEAVGSSTEESLSADALASMLSEDGEQSAVGTRYQVEVKETANDSVRQLREKAEDQTGFPDWYTGESPTYSGTSCSRDGFALMKANK;> MMRSSSFCRRQIRPYYNLPSKSEHGRKMTGFLTPYRHWMWKQNELWRNVHEAQFEHLRRVYKRQWLESFRVNADEYIYKYNITKAAQLAQWECEMKEQEKKRIEARQMMDGRQALKKKHLDLLREFHERQFFFWYERASERLQNMNLINYVPHAQLREHIDKELDKYVAGKNEPYPLNFVGQMPFLEDGDGNIVEVPESLLSNHMAEHPDSTAKPHEPHTSSSISEAAAFEERMLRAMVSAKEEDLKEWLGDDSRALSETIDDISREEEEREADIRVARSMEETDAEREVSRRAYIERGKTGSRSIFRPPTVSEGAGGTPSAPAGDANTPMRRRKKGKLDRVHALQAHQDELLAKLSSQGLKEGVDASSVPERGKIVQSRGRIRDKAVIPTHEVLMQKPELAAGSTPGARIQTKDMVDKMYHRGKYKKSGSGDKSDGEDL;> MRSKTLKKSLAAMYMRPPVTCYTDACEAPVAMWDGAIPLKETRKLKNGVPVRTVSRTYSHPPQLTPTQLSFNDINSMYCVGNDELIQFFPEGLGGRVFQTMPPGHPRGFLYRKETHLLNLFVDKVQHWHTKRSVLSSLTNGRTGFIVDGPTGCGKSALMCQVVHFARSRNIVTLYVPDAKVWTHGEWCWPSTILPGFFDAPDAARSFLKYFAVANRATLTSWKLRCTPKDLPTEQGERQPQNLYELCEWGHRAVAPASIDRQSVCVKFLMDELSEEKKLPVVIVVDGWNLFSHETHFRYPHPDFLRGLASFNESSTDIDLYPQELPRIPASRLSFVRGLNKMILSGDDPNKFFITCTTRDFKPFDGISGFPNVETDRFANSLDEYAPYDPEKDSHFHPIQIGNFDEYEYRSFLRFLINSGELAGLGWGPLWHASSDFERKLYKIGFLSGRNPQGVVDHYHQELVWRYDYQRTRQKQYLLKRRMEGMSRGASSGAVGVR;> MVLRRWFPLLGVHRVGYTHPSTLPVPCAQRWDLRLARARIFQEYIEEKAPGAWQLEDERSMSPEFKTFTGYPMRDMRPGYGQNLPDYIMKKRLPNNTHYELFARRDIPNEDNAMYGKYLYDMTVHGTSLPSTYRMHKDINKAQRNDRKLSGNRFKVLCSSGAKNPPSGWEPIPDATEEEED;> MLRCARVALRADPLNGGSSMTLGSKGSKLSPEPHRRRMPWTAAKEYVPGVVLNARDKMVLDGVQLLDIESIDRASQLDPLEVLRAVVATREYNISTGKNIFQLASQATYNGRGQRFYRKEWQEGTYDKYVTLSAIDFDRDGNKGTAYGYITFHGETTTRPVQVDFADVPGWYMDFVEERAVPFTGIVPPPPSIGTDVPVDPHSYRLKAYPYYDAPNPPEFVERLLKDRGVLPDTPTETADVDKDPTTSDGSVHYDGK;> MRRWHRSLNPALFGERGSGHYFSTTRARLQLQAQDRIICGTHGAGIVAHQTAVNSSDNPMLSSVTTAAPAADLSRTKPHEGTGTSERDPYIRTLHNQRSAAPESSVSQSHTVNAPTVDECEMLAERWGTMNYWHNDTFPRLVVFLKKLLVPDVSPLSPTAESLLSMFEKVVIPKLTSDEEDRRKLVSLWSETTLQAEAAVTKFLFQRGSFESMLHRIITDALEKMSTLALGGQEGNLALEALKRQTLFKRNDYIQKRLIDVVSNSAYLGYGDSVWQVFFAAVEANEENLLSDRATTDAIRAAWEGVMREDVVRLPDVTGVVALYLTLVCIRESGRLVPEELKELSSGLEDGVRPGVRKLQQYPLIFLHPTVKRRFVVKAVAEILHNSSSNAFSNMLRENGLHDTAREVALCEAMNRNKELAEGDVGDAVGRFVSKGEVKTLLSSLVSGTDAVVRDAVAGIFGIGTTITIDWDAVMQNVDWSNNWQRLATALLSNSAVLSAIVKLVKNAIGAKGMSKHLFTDEYADQLQLILDAREERAASRKQRIENIAQELSSFERVDLSCDLLRKLGVDMTELDTAAAATRNMNVVQRPCIEDGLLSLVLEAVTKRHPNWVKAGVIQTTLKDPFDALRWMMHIFIRLSYVPHAGAATIARLSRRRIGPIGLEPHQFNVPAELGFVEQYDNLQYKRYDWQGWYQRMLDVHNRNVSLRCRICDLQRLDGNGVQFVDMQTERRLRILAQHRVGMGVLKLDADKYEDQADNVTFGTTKLSELLADARKAQLGEEYWPSVELKVRKPSGQSKAHYSLIDNERIEKRSRELYEKYRDAKKRSLFVTPMETWLEVKGMQVRKSVDNADEDGYTLDALQDMMDGDDGDKV;> MKSSDIFFAYRLTPVVFKSRQHDSGVNQYGLKPTNAYDYINPTNLINFGRGTTFDNLGVRRAGRGEIDSSPSHSGSPVFTQAKLIGLSGEEQLTMCQSETMALRLCMAKAGKETCERESRALDSCLGRVGHLRRAMSEACWEFNDWFIQNVSDNHTKPFQHRPHDWRHFYAQEKLVRERQQNGHAYGRRPKQFSFGARYVKTDGYGKRPRLPYNK;> MRAGCVACSRIPKLGIAALGSTTTSMQATCQETQELRCATTQMAPAVIFPLPPPLRGSYIDRKPTAASFNEHHATASFRHHMIASADVSHRPRHFYFASGTRNDTGTRSVKEGERKQLKQQTNVEVDSVAYGDQLDELSARWAAKFYGQVTFGPRNYPYPSSRWLARRFQMKKHRIIKRFRFRRYKLAAVANLPFAKMIRVGMLPELKSSKTKRGDVVDPTLSGQLVSAVKNTGEKRKGQRTRPKSKYQV;> MLKRTLTVLDQTYGPHKSYKYTYMPDPRKLAPIETTQRSEIVPQSIRPPTSYVPNHETFLERADIHRLRPTSDFKASFKDWNDLFTCDKRQLRVRGIPRMTRDAIRTAVQAFQNGNPPERFDTKEEWLYYKQFKTVDYSYRVIPELPEKYRPHQSGIDQAPLPDYREINKMPQWAECEERRQSKKTV;> MRLCRRLSYHAYVPKGASVQMGETFMPSNIATAVFRETEAAAARADKTKEETGFFSQPRLNYPVSSGIPALFSKDQFDMQYSLFHRDVVETLNRHTLGTPLEGHNLETVIRKTSFDATQAVAHTAASEHFNYCFFYKSLRPWGTAPPPRLREALQLQYGTNGSADAMDEVRRIVWVTAASHQERCGWVYLVWSGVHFDVVEFPHGSCPIASDLIPLLALNVHESAYILDYGTSGLKQYVENYFKACNWPLAERYYLMAIGQVV;> MLRRTVTSLRNARELHRLLPALLPLLDPPVPTGASVCAAHLIVATGHVSKQREPHMSNCPVLERKIPLSEIASDDNFLKHPCVPCLKHRINFLASEDFCYDFVERCGCGTDGALPPEWRCIVERQFGSMAALVEELVIHASNRREAGWTWLVYDAQQAGERPLLVVNMPAQRSPLLLGLWPLAVVNVTEAVLVEAVRAESSGSVAAAPPPPWCRAARASLYDTKAAAEAFAMTAPMSEGVGKKLSEIREKVARDAVSRMNWGFILQQLKKAETYYASSDRGEKIRVHRMKLEREAVTKAMSGLRDSGATFLTHDTVEVTTTPSANSEPSSPERVPGVQAKQPQTEGMDPCKNKASAEPDPKCTQLPDGTWQYSYRNGDVTLLKPDGTRVFRKRELTTTAYPDGSMLFQYANNTSILDRADGVRVTTFEDGTTKEEMIRR;> MERRRLLHDGRWFTPCVLYGSARRGLKTLDVREYRPLAMPIEFRFYQRYANHPNRQSGIQFLTHYNTHQRFRVNKDYIDYMHWGKEQGQARLPHRHQRVAFDFNDQLHPTRIGTPEDGGNANHCYPEDGEDGSYAWFASQDPTFGHHPDLSSSFDPNYRVFSHPEHWNKMFTKRRPGEGDIDLSVLPSRSLLGPLMAHSDTKGIPYFKVDNRGHSNGRVPGVNAPFFGEFDQKMMQAMSRPLNANRTITGNDGRFSKTIMINEPQCNQALSAKTASELSKEIDKATNAVYSKLSVLEAAQSGLTDYFCGGLNFEIVGFELHMAAMLRERAAAILERSGAGGLPSASSATLSSSSTTRRCAMLLEKADEREVNKLLRDASRYEDRVDDALRQHASLIWRVYTAPRPLMTLTNGKCRGTGCGLSLFAKYCALKDSSEFIFDGPNVGITPYGGMTRLLARPETSLKYPGLAEFVVLTGASLFAGDALRLGWTDLFTTIPDMTYHIKEWFDTTEHMHNDAVAWQLGHLLETCFKMKESHSSAMERAAITPTRARWVEDAFADQPSVNDIMRTLTEIEQLPFQSTHNTSDESHITPYTLGSVAAGVQRLGEHRLRYTLSPWDITPPEDSVVLKHTSEMFRAYVLERRGATDVVTHRDAERAAAWSQQRQREYDAYCSLKEAPHPRHVYARLEGCEGKIVSFEFVFEISCRRSGPQGTDEVLQTTTISRLKSRILDALGMPRDRNIDLGWYLPTLDTCPIHSDEELMQVLHTDPGIEDPKEKLRYPPIYFIVKRCTLYFSEWAYAVKHQLLLQSPFALRAAFGLLQEVRGDGAAENVMPLAETLGTEFKYFTRLMRRPDFYRVGVHTDKSVEKWEEIKEERRHNIHHTHRPTRPLPDFEEVFERDVEIDGHRFVLRPRWNPRTLQDVDDSDILRLRAPLTYDMDSTAALHVPTHCGKASRLAGMLQDAGGVQVLDGLGEVDDKGEPKVPPLQSNASVPTNVSFYEMARHPWEDRASSWRRDGFTEGSLEYFESQYRSAERAVYDEEGRGVRNYWPSRDAVEGIAQEEENDAQLLQERLFNTLETAGTSVEPWARNLRLNATTGKFGYKTEIATQEEKIYDDEYYRWFIQPGRHPNPSGLTLNGRKGQFEEGHSRDEELERMWRKVVADGNNDFAATTSGMPVYDEDAKNAEDSYAAGDDVDVVTTDANVPVDGDDSS;> MMRRVASTGSNGGHCYVGSSLWADSVYMEVSSITLQKRFSFKYATKLQHDEMRQPYYIHEKRYGIFSNERNIAKARRGLPFITPLYTKHMNLWDTDTDASNNRFFRGYYYGQRELHQLLGRPHSLEATNADGSNDLSTYEANTSQLYKGIPRPAITNLHYEPAWRYTLYQAGAHGAQLSNPRSPFTAKVLGDELMQVRDIKSVEHCKAWFDRLQYLINLHYEAVGDIGEFKSRHTRHVHEFFVAFHDALSSLDFRDTYLFDQFKAVRPPELSDLFGIFLEMEANYVHEDYCPRCSLPYSTTRYCGEGDVDTPFRKHRGRWAPHQKWGREWYDVVARRAEALWYRATEDPYFGTPQHTQRQAEALLKVYVQAKQRGKAIDFMNKLRGSVEYLTGDITITTVMQESYDALLDTTPHPHLLTNGFTLESDAAKYTGEVNKAPLSPLQFRIDMEMNKYRRQQKEEGVVRVPPALWRLDTSAIVPYKVDSKTRRIVNWREVKEGIEKSFLSVGLPKEAYTGNEWREMLYLHDVIANREAKAAVLEQQQKLDREKLKARERASLKGEKSSNSASNGIGIIFPDKDGYQVFFVDEASLRPFGIGASGTLFKAVARVYPSPAAVPYDDPVHGKQFLIDTTDETCHLFGGFEHGDRLLLRAKSSGGDVDGGNNSNCRNTGSFTDEEEEVIVMGVSTEGSDAERMLCAMHVDTGKQRERGIVFLGTDCIDIRERWESVRYAASAYVKGRVTLLESQRTAREEFMGQVVGIRDGVLFVQWRLLKGGGSVLDRSVAVPIGDSTQVRELFVETKVLGVEPLQSPPSWRTPFRNDFAEERLKELQRAPFKREKYVSLIQGKYTPKVKKFGYTQHTTVDDFETKEYKDRLLSKQFFQNPQAFEVVPDRHERSVQFGGKWEYQRTHGLPTVDRNELENGWSEVEPISDGEMKVIEQALRDISGPRPGNFVKPPSKTKSLQLSESWWEPLGYGWEQHNEEQKALCDVTEQRLIDGSNLPFGGKLPPFGTSYGMGERMRAIIEDYSKGFGLGPHGHSPTHDTIHYNTLNAEGERVRDLGYTDALGRLFSEKLGDRDVHQWAVESCADGEADVRQLLLSLHEWRERGRPPSLLLANVLSKYLEEEIAAFNKGIPENAPKLQLETSDGTLAHSGSGGSRSGTMWADVDPTTFALHQASQSTRSTRCDEPFILHLVKRAKLGECVTNFTDTAYIAHLESSVINEFHLALTKLVGKGISPTLLAQKTGQLHRGSVRVGGNVVPFVKSRELSRLLERMGLTSESIAVITRGLANCPEQESVGDDFAVPVSLILSWDGPGSSGGSGSGDRRLNTTAARNEQQRKGSAALSSAIRQLSQHQKQRGSASGRGWQNEDKMVVHVLEELSLRNDGLVMDIQYAIRENKKNRRLRWEFVTTLLPVFGGNEAKVEQLYSDYCDGKYVPNITVAVEAFIAFLHNATQHPETYSASDYFDIDDGKSSTASGTGDQPSAGQYTTLKLLDPLEGPFVFDNVKVEYIQTVERFRRHGIRAGPVMAPATGFIAANCKSLNYFTRRQEEVVYVTNDSDQGLRRSLENSAYHKTIAANPALQYLLKARRGAALVETFNRFFYRTMPMLNFYQNVLKHYSETIQPLRQAAKSSTRGLARALESERSAAMEEFRRNSERYWRNIIEGRSVEQVVLANGESNRRTVGGGAGEQLQKPQGNRDAVRTNFTGEATDGSRKGQRQHQQPPLSQQQQHSRGEGERSAVHTSPRQGGSRGMADLLSKLNTPKTGSGVKGSTAKNTGNNRRGPKS;> MIRRRVCDGARLAPNIRATFSAVRYQSGLHTFIRDSKPSNFSSVRRSENANGDATASPGATAGENPASSGDWASHMQRELFGEVDPLGGQAHKDYYRDVTRGYSPQYAPRNFANGGAVAYPHIQSPYEYEEAAHRRVWLDHDVDRMREEFTQHRASLRSLASAQEREELLRSRAAEYQVANTVHESESVHPIQQLYNSGGTSRSALKQQAVADRYSIAEQHSPLPLTTGVDRDALDEAQRTKDRILNDSFTAENLLITHGLREKEKHDFTILQRTVRIPFQGYDMDRFLAQQKGTPYGAQQLPPNVVPSSMEEAQRTLRGSSATATPLVDAVAQKVYARNTVVDRPAIGEQLTEQIINIMRASRTTAEQQREEERAQRFGLGRQGALVQDGGPDQRTLKKHTNDERIVDAMLFQQNAYRKTPTDEHWNPYIRRSTENGVGHLLQNKFDIMRREDRLSKGEQDLTERNTIHYGVPIQQIVDEFVFRHRNARGERPLDYFKPFPNFRALRLNRMYRDVEGFSLMKQRPEFLEWELFTRYRQHHQQRRRLALLHGLEPVANETAQERDTRRHRLDEICERTPFDEREMRVNDDEMRVSVETLRSWFGVYMLPSPTVVNAVLGGSASVNLHLYHLADEMGTADTREHVLSSRYLNRLLLLESYQNRVGRGFMNHVVGRAPEPVVPHEQPQEVLRHFSAEERAMYEQHVKEQTSRQLGEWERAMKRRRWLTDHQQYGHVVSHGLETSVVDLSHTETGAVLTVSTKAYEQEIEAVRMKTNATIKVDGMVYNLLPNSERRVVPLTVQLDSGEKIDMTSEDFDRCELEAFPRNLNHALNYGIANYAYNRGNYVETQDSIWEEQTASGQEGWSPATHADGLREGLPVRARRPIFSSSAEQRIAGGPQRAVIIQYHHQPFFNPEPRLVKVAFQCDGTIMEVPISDVMIWQRRYHGPERTVGDESRRYNPAAMRRYVDVTDPFNEKTSNTEHFLDKYEPKRNADTVADKYRTTKQITEIDKWTRYDSARADNYRPLSISHRRDYIRMGYIPRYTPWEWIAIQEADQPLIAEQIRQDNIGTSYFFSLNRYWRYKASPHGYIRHFENEVRDLLQYVDGVTPWKQAQKIRTYWEVRSHHPMPQFNRPEVAMHRNTVGLLPAHMWETDKKTGKVKSVKDSVRDYQTKTPYPKWVQL;> MFRVRRLAGFIQCSPCGKMGPLKQQTRRYTPIWKSDPAVDNVAPLRDEDERRALWAEVGPISDVGSAVTAWIRFGNDPVLHTAVPTMLGGKFRNQQREKESLLPNSSSPFAYVEDYMGTNLVFGSPVHAKESAAVWATYFERRYASRLRLSRRTVANYVGLINSPEVFDDESDRPETRWSQDTFFRECAYLSEKFLKEKVSNMQQFEAALKRASPEAYLAFFDAFQQQTQTQIPLPSPSVWHYEGERRKQWAEKFISISHKAQAFFKDVLSEDVKKYQEVPGKLLQKVKPVLADVGKILVKRHERWLKGRVWTSLTEEEREAYCMKEVKRQQMQVEDGEFDPMMEDDVDDTELEEWQREHDAIMKLMNSPIDGLHFTTLELWLHTMRCEELETEHIYTSARVRAIQVAARKKLYDTTSYEEVIQAVVESIARGTLDLGAGVLRPHFNEVWCQLNYAKFGSSTITQHTTTSRRQLLFFHAGSLKDIAATATLYYATKPLSNSLDYASPYKYRRSLITLCSNYGVETAYTTQRPLLRSAANLARAEDLIHAVVTAAAQPFGERRRAATRDLHMEFQRLAVPVERVIVANPVSALLESGADPDEKPVEGEKVNMWPLGAKRVVLYKWSAPNVEKLKAMESDAASAVSGSSLTAKRLREIQELKRRGFLEVSLWRRVTAQERKQRNEIVEAKKKQVEEVVRTVPSLAHLHQYATSLYSRIEERVAFPTETSTVTETTNMKEETNKPLEDSEWEFAVLLDDRVLLNKEESVELYLPYRDANGELLAQGEYRALVRAFDLEANPNLHPAYCSVGYSESFQVFDALPQLIAQFFRVKDATAEAAGVTHIPAADFTPFCAFLRDAGLDVPLRCEFEAGQAVTTDGDVYMDYFLQLLRGEAFHQSHAQAGLTEAQRAIEPLCRAHWVVHHPGADESEWATARRSVLDHAMQHEREWWFPNEMLDVKDVVTGSTNGLTPQMYPAAVRYGVELCTVLTAEGKFVDERGSGLSARCVVNGTGAAESVVFDTANCNGTNTTSVEDALRVAHGALRSAQDRHNTLAAFRLGPLSKQSQVLLFCGVNAYEFGGKYARTYAYAFEKAKKELEATAASGFMAPSLSHEDTERLSDQPTTSPSVDRFASTTHPEQRKAQFVPRVGPGSTPLEDPAADQKSEWS;> MLRCTVVGHHRSGKARAFVFRDPSLRMMRAGSGYQQLRRMGMPMQVGMGWRKVDSFHANTQYQHAWPLLSHDDLGNSDQSNNTKNIMYSMYMPKRNKGTAPWFRGADTYSVKYCEQGRYEYQRYLMINRFPSEYKKHFLSFLSNIRMSSGSATIPQEALHWLLRMIVDNFNPQHVHYIAAMKTLQSAGELDMARDVWKIMERQQTWPCTATICAYLDVCVEAGEKTWAMEAWNRYCTELKFLEPGEVDPKPISRVPFSLTREELLYLPKWKKHFDHDPNLDVMDLNRFNRTREVYLRMAQVMLAGGERNAFQHFFTKLEEAMLNKPTPVPEPPNPHLVRRPRWAPYEHCKSVHHSPWRLQNNGRALALGPPVTIEDEMQSRFFSNDQFLVHSVKEVLRIVLQEHKRAHPTECTRCKTEAFFYKTKDADETLKFCDDLIERLFASLGVRLSNLNTSSLLSTILEVFRVVGKESGAALLQRANEFLERKASLGDAEGSRENLTASNYLQVLSGFADESAFVYNTKKDGTCQYKTGFDPRTTMRHLADVVQEIAGNPHVTWAADMHLQVVETMVGCGTMKANDYFVRNVLRQFSWDSRFLEALYVEYRRQDDVDMWAELTKRALVWTARYNAPASERLRRLIEDDYDTIRVQTRTFRELAVFQFRDVEERRHSRDVVNELPNPWYDYVAHALPFPDRDAGYPDEYGDLGQWRAPGGPGSPVRGPGYYAPPMEGEHQRGYTAEWRDLRNPMRPPEFPTPWERKYRQYARGQHPSYDMVYAGPMPEIFPMRRDFRKPTRWDFHDIEKQGKYRTSGPY;> MRRCSFASTCRYRSADDVPLGLGSAYVWTCRNITSRGQFNPIHNFSYAMERGVRARDVKAFEKLITNPGPLRVAYTPDYLDWLHRCYKAKGTYMDARAVAEKKFNGNIVSSELSAAVNRREGKRGDTRGDTVDNDHHNLPGAPPPGMFLRPAHSFRRLAGELKRRRAQSILDEVARAQGMLDLFERQPHFPAIHIDRCSRFHLVELFKEMVLERSLDSNMIWEKALLYRAILSERKPSYPTSFHYIFTAVEDTVFAPTISTPMEMAGSGGEGHDRSSHPLAAKCPTLEAYYYYVYLVKKYYIDNAVEAHVVLRCHREPNAADLLFSNPPPKDDTEIMKAVELLRNADIQRGVAAAAAVSDPTLPPGGEGSVIGNSDNXKNSEKXSEGSRGRPARPPVLPGAYPPIDMLWRCEENLPLLKVLLFGEFNLIVSENPFVKFPSAHGFLTRPYSTDSSRTLADGMSLANVMAEKRGHLLPSLPRNTATSIDARAQDIRRLQQKHHRDDIVSFQKLLRTHAEDSPSAFSSYSDWSYFNPRAVRAEERDRLTRKAVEALKLYDSATNDIYRHSFEDVQACHTQRVTERDRTMPPYLPTLPHFVAIIKKDPHISFLLHIGLPDRNSSEEGSAKHKELEKRIYYLARALYHTALEYHNETVRRVNRQKVNVAASLLDNFVEQEWTTILRDKHDVTDVTKTLNDTQNDKKQLARRLGRYMLFANRSLDDTGFPTDARADDYTRWMAPPSVGKVSL;> MSVSGVFSKGRGIGHEATTSILRYIPRARVPWQPSRFGRENLTAADMARLWSRGRYRDGPGNYNSGYCTERTHVLEENTVSIIPRRELEKYMPDITIGPKALVTPVSLMNARNGHRVTHDLLHSYDPHIGRLGKPAVVDHDNITVEDPNRVGLNAATLDCRGRIYRWLRRGPFFQVDNYFRRSVKLNRDGTLPTDFVHEAPLMRKIIRLAHRGHLKAACEEYRRVTTVPPVEVYRALTACCVPGAKLADAVSIFEDGDSKLFYVSRDGEVLHNLMRCAIAARHRARIMWVYNVMRGRFYENVVVRAEVDLIWRYRIAMIALEYLLDHECAEEAAAIYSYLVEEELLRCDVHVRVGLHMREAIAAGKPITLNNDVMNATSLVRDATAVAPEVARELQRRHAQTLQNNAVEAVGAENVREGSAPWSILGPLTAIGPTAEDTMVWLQQHYGDVDVMSIMRWARFRKGKDLMAKDRPQYLARAAAWIELLSKRNREMEEVPLTYMRKSKPLVLDTNSNVRVAWQTPLMRSGGPPRLLAREEGYVFHHSNSSRFVEETYRHPGESLQSRYLALQPLHTEVSAKEDFQRLYYQAQKHHKQQERLLPVSTAAIPSRIVHHSVMSALHGVSGKGEPANRSLFTXNKSNDSHSNTGVASGTSACTDGAGSATPEF;> MFRRAIPLLSANIPRSVWDPAQHNPNWSDSYGHDITNRRAWPARKWTVGLEPCTPREWLQFSHRNLAYAYNGALRACHSLPSMLLLYKEMKQRGVKVDVDTMNVLLTRAARHEHIQVDDVFLLFDELVALGARPDLAAAETLHTVLSHSASMPEEWREARRLQLVELYNNLAMEEVERLAPHRADRLLKEQMKRFRGNLQQLGSGLRPTVYCRYLHTTHTAAVLLEEVHNFLWELVPNDHPAMEIPALQLRVPFVASVLRRPSVNPGVSLASVSRAEFGDTDVCAVFLAAAERMVDADFDDQRPVSERRLFLSLLTMISYSGVLYTSDLMAQLMEMVKYSNNDETRDSDAQRVLRYALRGSSAAQDSASRTLWHSVEKVADCRVVGRYIGARNPWNPIRVCFDEQGVFKAYPISTTTTTREVSPPEGNGAVTQEQRASCVEGRTLEALNMRWDDVRRLIECTGVLVTPPSERCPQQQKMEVFTGMAVYLRTVATGRRYEGGEDVLSDGAVATSSCEQRRRGTLFAEGYDFDVWVRLFSLVQEVRHDMEKFMADHTLQCVEPEFECWEALLVTLRCALDFCVVQMQGGGARGTEREVVERLFRDVVALREELIEESRTRFGGRMRVLWLQEA;> MLSQNVAKTTVPSYYMIRTNLPHRKPQNQWEGVYYYSGITKRQRHLILLHRKREREAHMRSFNISRASVLQRLEQLSGDRKQESLPPHVRLDLAVRLAQHGLYQQATPIVDELHHQKALHAGHYALLINALACPRLGQRILHCDAQCDPALTYKLLGDENGEERAQEAYRWFDLALTSLAVDCGGRTQPSHFVPYLPQGTAAASHITNALMRTLLTCGYTHVAAIPDSVYDRMGSMGISPTISTYELVMLALSLQGNMVEAESILSFLRSHHSEHITVESFNALLLGHREARQFDCCDAIWQELVDRRWPRASPLTAELYLRSIMDHANTPTSEPLQSFANINVVEKKKVPLVLAQMDELGVPRTHLSRVLMDEVEDSLRKFQTYRSRFYEWGRAVKQFDFIEFRRRNGWLYDLHLMKCTTKQVGPLRDFNDPDAVQGAVATAEIPAFFNERPAWERPPLEETLYVTTNKERYDDVRGGDIYYDDTRGLHDRSPTWMNEVPETRYDRLYGVNHPDIAKIGIRRHLNVEYVNRKEVVERDAALMKKTLSSGRRLRHRVESSRTHRNAGSLSGISSTAGGGSR;> MRKFCHFMANCWNSARSHATYGAVPLTHSQVTSVYATDGGKVDELGLLELVEERIFSWKLNKWEMRIPPNLPNDQKELIRQEQENLKQILSEWRKCFGALNADILQISSLTGVPKDVVREKNRTWLQEEVAKLRWMGEVNKAALLRDAFMRLEAFGSRDFMFMERLCCIYGLARQGTFDEAFTNYITEDPVTNDIFVDERNPFKELVAHIVRNYSQIDIIYDFLGFNYSEGYRSSLRRYMEYLQCKTAENVRASGRLVTGDKGEHNILFDYCVSRESLVSGDSCQGIIDFLYINGNDVTLIIIASDNPWLRNRQLPHRRQMEGIARRVCFVLGIPPSEVRIRNLLLPPTYLDKGSIVRLNDIVFRLSNEQSNLLIPWLTNYNKELDPKDVDYTALAKTTNEEEWLTL;> MFRSTRPRSVGYTPVNPDTSPMVAYSQYHWHYNLPQGMERPHSVNRTFAAPFQSNHSLVNKYRGVWIEFDMHPAFSVALEPQLRKLPRGRTLPKTPAEEVIADYTALAPLVDDEKTRDLWLAKVFQHCAFQRCGGAMELWERYCHQRFTAEGATAKPPLSLVKSVLFYCNKTDNSGWRALFDRCLKDGWNYTPLFDTAQWSFMLKSIGRMGDEDGVRAVLEEMLDVQADLDRVEARSVVIALNAVTNADVYEFVKKYLFNFGERKVKFLRTTYSDLRGHGAGKLRIPLKENDNMYYHVCWHSSIRSPRQFSPRQLYFDYTPSTLGSSSHNPNAKIDDIVKDKIEKWKAEGLLPEDYVHEDRVYDRSAAFKNVARQEKWKKMPKILKSKRMGYTGDP;> MSFRYTNNLIGALKHRLLLESSYREIASRKFIGNCRGVEVVCSGYGTVLAVQLTDKAVWESFYRKGGRPTVSGGGDVSGDAETGTQGSATTTGATGSLDLDKLAESIKTALWDATRKIRSAKEAALHRSLSHNTRMRASADLKHWYEEDANTLRPLAFEALKHEAATPWMQLVQHGKKEEAAALLKEFEQKGDAAEATPTRVKDDRVKGTRTELSNREQPPLASTLKAEDSNPATIPIGSVHPLFTPALVQIEEAGGGSVSNEAVCRAQLWELSRDEQLFWERVELIRKGQVASIGSSHKRGYADEAAFAKDDTEEKVQLRFTQ;> MRCSCAFLDKSVFAAKRRVIVPIHPTPNFPAHFIKSAFTTDPLKEKQKARFSSGGEAMREVQDIPKNLEGERSRRDLASRGDTEFQALVEFIEGASYDQLISGRRFKKVYDVLSENDDMFIWLCHTAMSVLNPGDMRSRLIYNHLRILAESVASGEMTQRTAFRFFESAVRSPAYREIAKRQLEGGAATRLAGISAAADVMRRMGLTRRPMSSYFELYQRIVERSEAMTPWGFPPLFQFEERLSLEPRLKFFSRASQQSLERRRRGHVMTPHTTLHGRRIFWIPPTWNRAGRFLGPHVTLYPGMTPD;> MEVYRRITERVRGALWAHHGRLMSERQFHRILAFVYNNKYEYQIRFDRMEVVGREWGGRVEVVTTPAGFLKRVRVNPCVEDLTLYQQQQLILSAYANACADGRKLMEQAEMNIYKQFLKDLKPIVMGIRDNPEFYTVSENSIETIGGVLQTGDSNNLCHTHRTIPAAKARQPADEVRARQEWEQKWINSPRGQSWALTLRGKTYFALHGPQYRPRGAPGAKKETLPLDIPAPYTAMDEKRLLKKNWMAYLDNKHVAEVMWTRVKIADREKRQRLLQETGRAWHRPINEEAINRW;> MLCRTFLRQFRMSGGDMFVEYKVLSRDHRRSIRVEDAIVDPTFKRTVLPLGWLELLRSPSLRLPTGYFVEETVHVSLPNATSNGGKKEARPQKGGFASGSPSVGRNEANAIIAGPVVLYITGQSVPVVLNPYFVPEGTWDMRTRDGELDLRLGMDAIEQCTLFSELRPGGLLYGKLPENPNVRRNESLRATLGRYGMKCDLAESPLVPRPWTRMRYMFIDELQRGPKLTEFVGHNPRNGTPWRFSQNTKYFRIGIWRDTIRRNDMNEGLHAHSSWQKSPQQSVPEVRFLAPYP;> MRRFCTARVSSYVKRAPLLLPRGGRRWRSGAGTTADGGGEKEYIADSFESTAGSNAYAAMELAAEARREIHELWLSAETALEREKRVQQVAALIEKYKLDPSTPREADVSRGLGDAFDRLLLLCLPLGKTDAKGTDNLERLMHLAGRNGRELSVRTIQHLFARTDSFAEALAVFYTMRRCHVAMNMEAYYSMLYSLQRLEEEGWGQHFRNEYEENGAPSEQAMDFIVKGISNALLPENKPWLGRVMFQDRNVPDRRYDTRDFDELDTAWTQRYKSGTPAGAH;> MLHGTPVRRASLRYRRPYWMMFLKGVDNWKIYTVIQQPDHQRTEMLYQAWLGGLDRPYTRPKCMANQPLWLSKKRHMLRKERLDGPETPLEKYVLEWHKKFHSFQGTERPTPDDLHTALDLVERPLDLSYALQLLGQCRNLNNIRFAKETFLVFLEACLRVGRRDCAEYALEHAEPLGFWFIDEDHRRYLQGEQTWYKLSPLDNLYYPVEENAKLNEGRKPITRLSPATESPGSGTAISDGEPSTDVEGETTVDDEIAQLEAELAALEREGGGK;> MLRRVPRVLQKGERGLYFPINHRIVDHRIAPGVTVEETDVQSRYRRELRTNFATGETRQTIAPPWSARERPTHFFSLRLPSRNSVTLRVKEMHNHLLFSHQQCAPMLVSPTKLHITLGVMTIPENSREELVKNIQQSMSETFACVQPLQLRFRGLGTFDFGRVLFIRVVPEADFGRLERAVCDIRRRVGGVLGVDLKGNPHDSYVPHVTVAKIRPNQRQQLGDTIPQSLWADYQHHDFGDVTLSTVDLCRMKGSPDGYYHTEGAVHLS;> MFSESLCILSRRFRYNTKFPALVSYNKLPWEVVNHETPQFHMHVAPHYEQLLTLAASSPVPHIIGSKHIDVPREHRLRLLPGMLYLLDGDTLPGEFTINRVLDPTALQYYGRLSSQIVTVEAVRMLVPDDLRLLCNCITFKGPLHLPVAPYASLASLRGASQGGTTGSETGSNCFTLYHFVRPNRPPKELQLEKYYIHAPCVAPLSEFASNSDERGNWRPRLQAPKRTRRATPLPAYRPPQSYLMGLAERLAVVPGGCFGRRSLMWGHWF;> MFNRNFILRAAEFKQKSRWSSVWPNMRYGSMFLSYSVGRKLPMKGVNWVTRDSNRLLNFSNRYSAVISDIDVKRTEEELNVALSDIRWNDHRRIYWKCSFCGSSYRKNVSVRTKYHAGCNFCKKKYPSEVRGEQHGSPPVSQAAPELTEQLVDNGKRDNLATLAVTSKFYAEWTCRGCGGSYRSTIRSRTGQVEAGQCTLHPDIVAWSAYCPSCSWRPNMVPIAEEVSRSGQFLGLERSMEELGGQRGKQLPIPRRKRLAC;> MLVSYLRLQADRRTRHHMMVDGQINPREWFNWHPKEYQPWYFDRHKFLYEQRQYAQFHHLLCHQVYLKDMLHLMRYPEPYTHIIDCRTSTQKMHRWVPHSLWLPRDEVEYALQLSADEFLDMYGFRKPDKSDDVILLSHNGIYSEQAGWEWKKQFFQHVYNYRGGTNELFGESYSDMNVSDVLSPWKGPFPQSGVFVDKWSKRKVLTRTGPFDRQYEMQDFALPDLELEKARHPEEGPRQNMPFGLQ;> MRRGALSLLKAGLLGHYQQEAFEARKRFEESTTYPGPIRAATPGDTRFYSGSLESILHDTDRHYWRAVTDDPRVQHLIPLRIRFKIFTWVTSGWEQRMQVVQIMAPKDSTIAQVKDLVIVENQSPYLCVSSFHLAIDGKELDPQKTLGEYGITEQSQIDAIEQNDHLLHRDDERPRDWTVDEITAEDVKRSPYKEMEMQPLQNLAPRYEARPKGYFGRTYYSGMKQSS;> MRRVRDGLFLSHPSSALQCSVAVVSTGEFDHPPFQFRQRHTFNTTPLHDANRFGGRTAYLREIGPVNIKKQGRRFKKDPRTVQFNVDVWCAQQTLRKRWKQRDWEVIEIPFRLVPREQQRVIPELYTDIPQMTDPARNDFSNIRNKVYDREELQGVLFPAAGAMLYPPLQRVDKQAMTLDKYL;> MLRFTHRALTATPERFSVLGTTHPKPKRTGFGRNNKMRSKPSDNVAWYDKGPVEWLPRPVRLTYDHLDQLQQWTMRATLDGRTEEFNRIRDLHREWSQHPLMPVLGDVEPKFPLNLFKQNHRAKKRFLVRWHKANTPANWLWMPRGPTVVTPLHRTNPTQYPENWKQMVQRKSGTGTPS;> MFHRAFVSSSDLTGCTIALSSVCTQKRYWAKPKKRPKVGQGFHEKAQKWREEYLLDRHRALADSLRAYVEFSTSKRVEPWDARFKPFDRIEKDGVYVLMRYMMEEKLQLCNYHHRPVKRLFCNIGLMGPQITTKARWKPYRFATNPAGTSKAERMYQRDKTVYTHGHND;> MLRSTLTSLNTFLTSSVATPPISVIRTGPKWWADPERMVRQKLMYFTLGVDQLPLRRTAVIQRDLQRFHMCKPPPRVGDSTGYKRSRAAQLNTWYRRIQYQEYHMQHLFTRHVWGLLRVYPGNTTKIQGKADDGYVGYDSVPFHRYNRAPLPFPARELYERRK;> MLRRSILFRMKYADLELTTRGEFPHGMKEPAFVKKLDQNIPWYFSTYRSMYHWPITGDNWSDLNEAEKHHDLHMFYTLAWWKLGEGIFGVDEDS;> MFSLTQTWLIAHWYCGHKFRHRFMRDKRFHPSLQASHDARNRFSKRRHFKTNRWNYQQAYRDMP> SSLDDKPQFPGASAEFIDKLEFIQPNVISGIPIYRVMDRQGQIINPSEDPHLPKEKVLKLYKSMTLLNTMDRILYESQRQGRISFYMTNYGEEGTHVGSAAALDNTDLVFGQYREAGVLMYRDYPLELFMAQCYGNISDLGKGRQMPVHYGCKERHFVTISSPLATQIPQAVGAAYAAKRANANRVVICYFGEGAASEGDAHAGFNFAATLECPIIFFCRNNGYAISTPTSEQYRGDGIAARGPGYG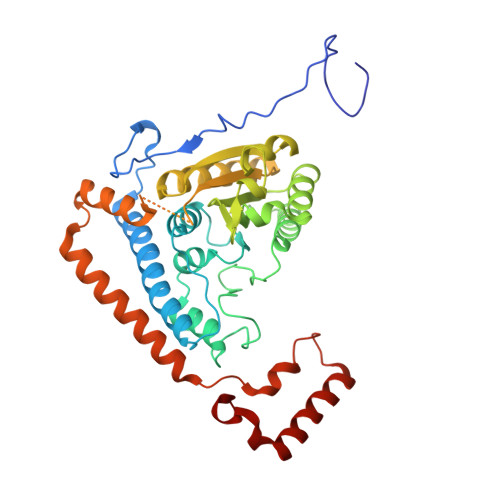IMSIRVDGNDVFAVYNATKEARRRAVAENQPFLIEAMTYRIGHHQTSDDSSAYRSVDEVNYWDKQDHPISRLRHYLLSQGWWDEEQEKAWRKQSRRKVMEAFEQAERKPKPNPNLLFSDVYQEMPAQLRKQQESLARHLQTYGEHYPLDHFDK The design of proteins that bind to a specific site on the surface of a target protein using no information other than the three-dimensional structure of the target remains a challenge. Here we describe a general solution to this problem that starts with a broad exploration of the vast space of possible binding modes to a selected region of a protein surface, and then intensifies the search in the vicinity of the most promising binding modes. We demonstrate the broad applicability of this approach through the de novo design of binding proteins to 12 diverse protein targets with different shapes and surface properties. Biophysical characterization shows that the binders, which are all smaller than 65 amino acids, are hyperstable and, following experimental optimization, bind their targets with nanomolar to picomolar affinities.

Unlike antibodies, the designed proteins are soluble when expressed in E. coli at high levels and are thermostable, and hence could form the basis for a next generation of lower cost protein therapeutics.

> GGGDRRKEMDKVYRTAFKRITSTPDKEKRKEVVKEATEQLRRIAKDEEEKKKAAYMILFLKTLG>SHPRYQQPPVPYRQIDDCPAKARPQHIFYRRFLGKDGRRDPKCQWKFAVIFWGNDPYGLKKLSQAFQFGGVKAGPVSCLPHPGPDQSPITYCVYVYCQNKDTSKKVQMARLAWEASHPLAGNLQSSIVKFKKPLPLTQPG[10x]

Latency associated nuclear antigen (LANA) is a 130 kDa multifunctional protein required for TR-dependent DNA replication and episome maintenance during latency. LANA binds to TR DNA through a conserved carboxy-terminal DNA binding domain (DBD). LANA binds to two adjacent sites in the 800 bp GC-rich terminal repeats, referred to as LANA binding site 1 (LBS1) and LBS2. In this capacity, LANA acts to form a site-specific origin of replication and as a molecular tether between the viral episome and the host chromosome.

To characterize the structural properties of LANADBD, we crystallized a construct encompassing residues 1011–1153 and determined its X-ray crystal structure at 2.05 Å resolution. A comparison with the DBD of EBNA1 shows that the two proteins share the same general fold (RMSD of Cα atoms = 5.1 Å) despite sharing very little amino acid sequence homology. A central, anti-parallel beta-sheet forms a hydrophobic core through which two proteins subunits form a dimer. Three helices, which contain the key residues involved in DNA binding, flank this core region. Remarkably, the crystal structure of LANADBD reveals a higher-ordered assembly comprised of five dimers interacting end-to-end, forming a decameric ring with an exterior diameter of 110 Å and an interior diameter of 50 Å. The dimers are arranged such that the DNA binding surface faces the exterior of the decameric ring. The interface between the dimers is small and hydrophobic, consisting of residues Phe1037, Phe1041, Met1117, Ala1121, and Ala1124, and buries a total solvent excluded surface area of 963 Å2. In our DNA-free structure of LANADBD the N-terminal portion of this construct lies across the DNA binding face, based on homology with the EBNA1 co-crystal structure. The surface opposite to the DNA binding face of LANADBD is a dense basic patch composed mostly of lysine residues. Consistent with this, the angle between dimers in the decameric ring is approximately 110°.> ETGDSIIHIGAIFDESAKKDDEVFRTAVGDLNQNEEILQTEKITFSVTFVDGNNPFQAVQEACELMNQGILALVSSIGCTSAGSLQSLADAMHIPHLFIQRSTAGTPRSGCGLTRSNRNDDYTLSVRPPVYLHDVILRVVTEYAWQKFIIFYDSEYDIRGIQEFLDKVSQQGMDVALQKVENNINKMITTLFDTMRIEELNRYRDTLRRAILVMNPATAKSFITEVVETNLVAFDCHWIIINEEINDVDVQELVRRSIGRLT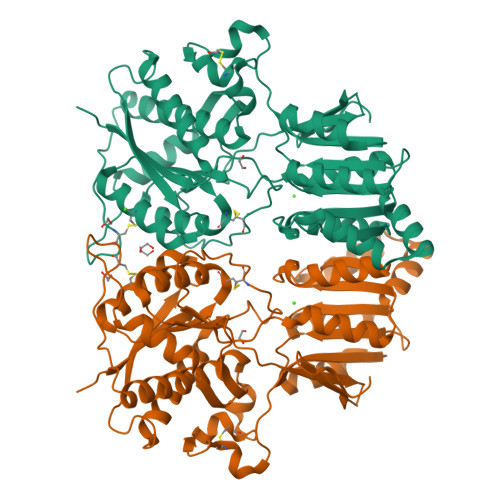IIRQTFPVPQNISQRCFRGNHRISSTLCDPKDPFAQNMEISNLYIYDTVLLLANAFHKKLEDRKWHSMASLSCIRKNSKPWQGGRSMLETIKKGGVSGLTGELEFGENGGNPNVHFEILGTNYGEELGRGVRKLGCWNPVTGLNGSLTDKKLENNMRGGTKHHHHHH> PYVEIIEQPKQRGMRFRYKCEGRSAGSIPGERSTDTTKTHPTIKINGYTGPGTVRISLVTKDPPHRPHPHELVGKDCRDGYYEADLCPDRSIHSFQNLGIQCVKKRDLEQAISQRIQTNNNPFHVPIEEQRGDYDLNAVRLCFQVTVRDPAGRPLLLTPVLSHPIFDNRAPNTAELKIC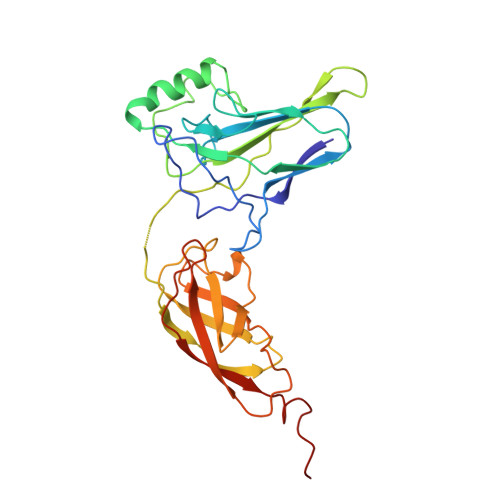RVNRNSGSCLGGDEIFLLCDKVQKEDIEVYFTGPGWEARGSFSQADVHRQVAIVFRTPPYADPSLQAPVRVSMQLRRPSDRELSEPMEFQYLPDTDDRHRIEEKRKR> MASGSSHHHHHHSSGENLYFQGHLDLSKDSDFQAVEKQLTKDTNISGKFIQIRQIAGLNSSLKSSGTFKLTNDGSLLWQQQSPIKTTMQMSKNKLTQTIMDNPPTVLTRDDQPIVFTFTSVFMSVF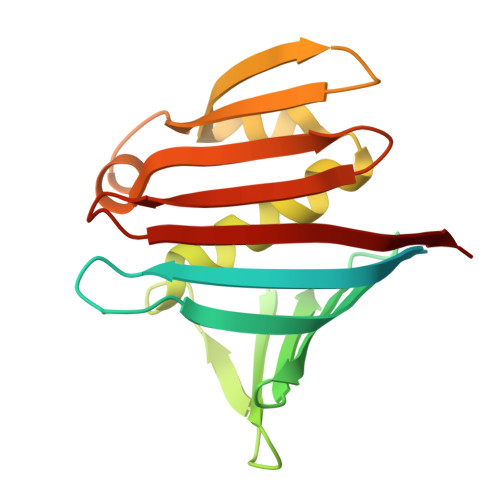KGDTKTISEFFNINFDGNTQNWTITLTPKSSPLNKAIKEIILKGNRYITNIDVADTQDNIIKIELFDITTN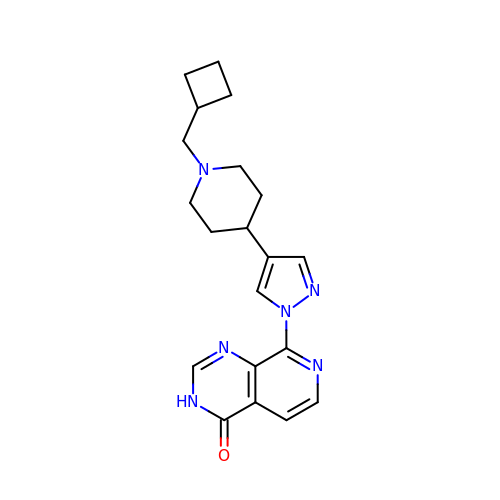8-[4-[1-(cyclobutylmethyl)piperidin-4-yl]pyrazol-1-yl]-3~{H}-pyrido[3,4-d]pyrimidin-4-one | C20 H24 N6 O | FQYVJQRHNLIPIK-UHFFFAOYSA-N2-amino-1-(3-methoxyphenyl)-1H-pyrrolo[2,3-b]quinoxaline-3-carboxamide 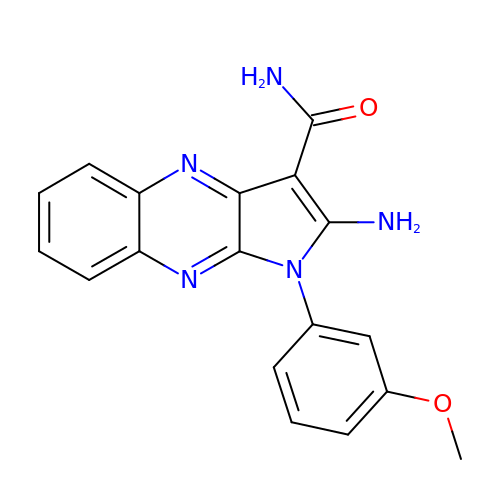| C18 H15 N5 O2 | CHHKMVNVTYIPGZ-UHFFFAOYSA-N>MKKIFMMVHELDVNKGGMTSSMFNRSKEFYDADIPADIVTFDYKGNYDEIIKALKKQGKMDRRTKMYNVFEYFKQISNNKHFKSNKLLYKHISERLKNTIEIEESKGISRYFDITTGTYIAYIRKSKSEKVIDFFKDNKRIERFSFIDNKVHMKETFNVDNKVCYQVFYDEKGYPYISRNINANNGAVGKTYVLVNKKEFKNNLALCVYYLEKLIKDSKDSIMICDGPGSFPKMFNTNHKNAQKYGVIHVNHHENFDDTGAFKKSEKYIIENANKINGVIVLT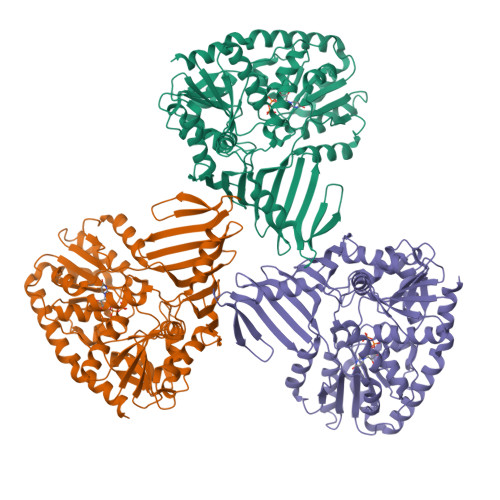EAQRLDILNQFDVENIFTISNFVKIHNAPKHFQTEKIVGHISRMVPTKRIDLLIEVAELVVKKDNAVKFHIYGEGSVKDKIAKMIEDKNLERNVFLKGYTTTPQKCLEDFKLVVSTSQYEGQGLSMIEAMISKRPVVAFDIKYGPSDFIEDNKNGYLIENHNINDMADKILQLVNNDVLAAEFGSKARENIIEKYSTESILEKWLNLFNS[4x]> AEAGITGTWYNQLGSTFIVTAGADGALTGTYESAVGNAESRYVLTGRYDSAPGRGDSVGSGTALGWTVAWKNNYRN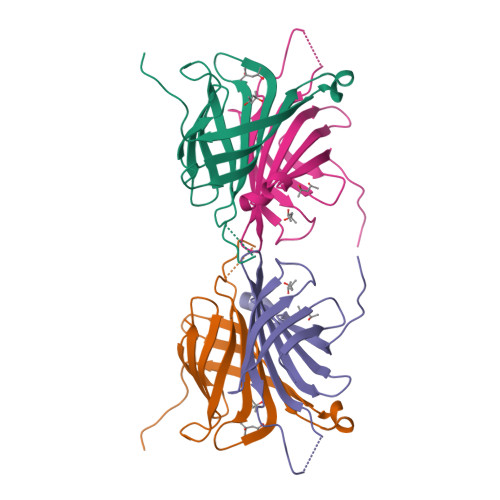AHSATTWSGQYVGGAEARINTQWLLTSGTTEANAWKSTLVGHDTFTKVKPSAAS2-methoxy-~{N}-[2-methoxy-5-[7-[[(2~{R})-4-(oxetan-3-yl)morpholin-2-yl]methoxy]-1,3-dihydro-2-benzofuran-5-yl]pyridin-3-yl]ethanesulfonamide | C25 H33 N3 O8 S | 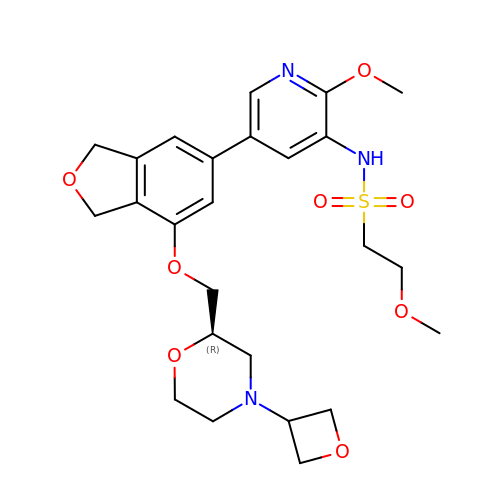ZWPJBXLFZFLGMV-OAQYLSRUSA-N> MDAKARNCLLQHREALEKDIKTSYIMDHMISDGFLTISEEEKVRNEPTQQQRAAMLIKMILKKDNDSYVSFYNALLHEGYKDLAALLHDGIPVVS;> SMDEADRRLLRRCRLRLVEELQVDQLWDVLLSRELFRPHMIEDIQRAGSGSRRDQARQLIIDLETRGS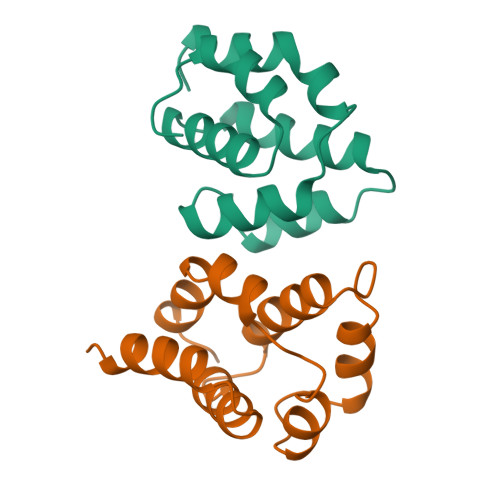QALPLFISCLEDTGQDMLASFLRTNRQAG>[2x]MTQHFDLIAIGGGSGGLAVAEKAAAFGKRVALIESKALGGTCVNVGCVPKKVMWYASHLAEAVRDAPGFGVQASGGTLDWPRLVAGRDRYIGAINSFWDGYVERLGITRVDGHARFVDAHTIEVEGQRLSADHIVIATGGRPIVPRLPGAELGITSDGFFALQQQPKRVAIIGAGYIGIELAGLLRSFGSEVTVVALEDRLLFQFDPLLSATLA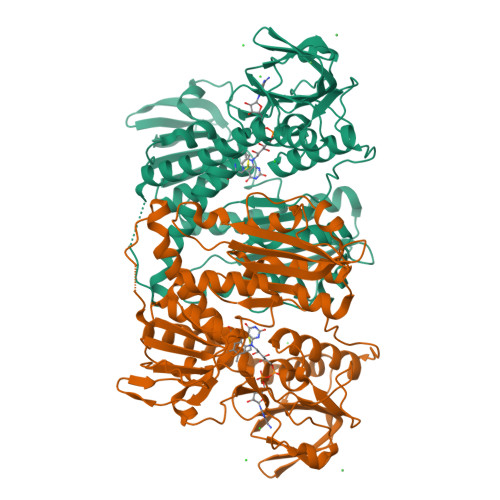ENMHAQGIETHLEFAVAALERDAQGTTLVAQDGTRLEGFDSVIWAVGRAPNTRDLGLEAAGIEVQSNGMVPTDAYQNTNVPGVYALGDITGRDQLTPVAIAAGRRLAERLFDGQSERKLDYDNIPTVVFAHPPLSKVGLSEPEARERLGDVLTVYETSFTPMRYALNEHGPKTAMKLVCAGPEQRVVGVHVIGDGADEMLQGFAVAVKMGATKADFDNTVAIHPGSAEELVTLKEPVRRPGDPLPEGAA> CTTTACCCTACTGGTAAATCCGCGACCTGCTC;> AAACGAGATTGAGTAAACATCGACGGATAGCTATACCGGGGGTTTCTG;> GAACCGCCCCCCCTGCCTCATTTGCCGCCAGCCGGCCAGAGGGTTACC;> GTATAAACGTACCAGGTATAGCCCGGAATAGGGTCACCAGGAATCCCCTGCGGGAT;> CTATTTCGGAACCTATGAGAAGGAGGAGGTTTGGCTGAGATTTTT;> TGATGATAAATGCCGGGAAAGGGGCTCTTCGCTATTACGCCAAGAGAA;> ATGGCTTTTAACGGGGTCAGTGCCATGACCAT;> TAAAGCCAATTCACAACCACCCTCAGAGCCGC;> CACGACGTCGTTTTAAAACGAGGCGCAGACGG;> CGGAAACATCCCGGAATTTGTGAGGGATCCCCATGCGGCGAAAGAAAC;> TGATAGACGGTTTTTCGCCCTTTGACGTTGGAGTCCACGTTCTTTAATAGTGGACTCTTGTTCCAAACTGGAACAACACTCAACCCTATCTCGGGCTATTCTTTTGATTTATAAGGGATTTTGCCGATTTCGGAACCACCATCAAACAGGATTTTCGCCTGCTGGGGCAAACCAGCGTGGACCGCTTGCTGCAACTCTCTCAGGGCCAGGCGGTGAAGGGCAATCAGCTGTTGCCCGTCTCACTGGTGAAAAGAAAAACCACCCTGGCGCCCAATACGCAAACCGCCTCTCCCCGCGCGTTGGCCGATTCATTAATGCAGCTGGCACGACAGGTTTCCCGACTGGAAAGCGGGCAGTGAGCGCAACGCAATTAATGTGAGTTAGCTCACTCATTAGGCACCCCAGGCTTTACACTTTATGCTTCCGGCTCGTATGTTGTGTGGAATTGTGAGCGGATAACAATTTCACACAGGAAACAGCTATGACCATGATTACGAATTCGAGCTCGGTACCCGGGGATCCTCAACTGTGAGGAGGCTCACGGACGCGAAGAACAGGCACGCGTGCTGGCAGAAACCCCCGGTATGACCGTGAAAACGGCCCGCCGCATTCTGGCCGCAGCACCACAGAGTGCACAGGCGCGCAGTGACACTGCGCTGGATCGTCTGATGCAGGGGGCACCGGCACCGCTGGCTGCAGGTAACCCGGCATCTGATGCCGTTAACGATTTGCTGAACACACCAGTGTAAGGGATGTTTATGACGAGCAAAGAAACCTTTACCCATTACCAGCCGCAGGGCAACAGTGACCCGGCTCATACCGCAACCGCGCCCGGCGGATTGAGTGCGAAAGCGCCTGCAATGACCCCGCTGATGCTGGACACCTCCAGCCGTAAGCTGGTTGCGTGGGATGGCACCACCGACGGTGCTGCCGTTGGCATTCTTGCGGTTGCTGCTGACCAGACCAGCACCACGCTGACGTTCTACAAGTCCGGCACGTTCCGTTATGAGGATGTGCTCTGGCCGGAGGCTGCCAGCGACGAGACGAAAAAACGGACCGCGTTTGCCGGAACGGCAATCAGCATCGTTTAACTTTACCCTTCATCACTAAAGGCCGCCTGTGCGGCTTTTTTTACGGGATTTTTTTATGTCGATGTACACAACCGCCCAACTGCTGGCGGCAAATGAGCAGAAATTTAAGTTTGATCCGCTGTTTCTGCGTCTCTTTTTCCGTGAGAGCTATCCCTTCACCACGGAGAAAGTCTATCTCTCACAAATTCCGGGACTGGTAAACATGGCGCTGTACGTTTCGCCGATTGTTTCCGGTGAGGTTATCCGTTCCCGTGGCGGCTCCACCTCTGAAAGCTTGGCACTGGCCGTCGTTTTACAACGTCGTGACTGGGAAAACCCTGGCGTTACCCAACTTAATCGCCTTGCAGCACATCCCCCTTTCGCCAGCTGGCGTAATAGCGAAGAGGCCCGCACCGATCGCCCTTCCCAACAGTTGCGCAGCCTGAATGGCGAATGGCGCTTTGCCTGGTTTCCGGCACCAGAAGCGGTGCCGGAAAGCTGGCTGGAGTGCGATCTTCCTGAGGCCGATACTGTCGTCGTCCCCTCAAACTGGCAGATGCACGGTTACGATGCGCCCATCTACACCAACGTGACCTATCCCATTACGGTCAATCCGCCGTTTGTTCCCACGGAGAATCCGACGGGTTGTTACTCGCTCACATTTAATGTTGATGAAAGCTGGCTACAGGAAGGCCAGACGCGAATTATTTTTGATGGCGTTCCTATTGGTTAAAAAATGAGCTGATTTAACAAAAATTTAATGCGAATTTTAACAAAATATTAACGTTTACAATTTAAATATTTGCTTATACAATCTTCCTGTTTTTGGGGCTTTTCTGATTATCAACCGGGGTACATATGATTGACATGCTAGTTTTACGATTACCGTTCATCGATTCTCTTGTTTGCTCCAGACTCTCAGGCAATGACCTGATAGCCTTTGTAGATCTCTCAAAAATAGCTACCCTCTCCGGCATTAATTTATCAGCTAGAACGGTTGAATATCATATTGATGGTGATTTGACTGTCTCCGGCCTTTCTCACCCTTTTGAATCTTTACCTACACATTACTCAGGCATTGCATTTAAAATATATGAGGGTTCTAAAAATTTTTATCCTTGCGTTGAAATAAAGGCTTCTCCCGCAAAAGTATTACAGGGTCATAATGTTTTTGGTACAACCGATTTAGCTTTATGCTCTGAGGCTTTATTGCTTAATTTTGCTAATTCTTTGCCTTGCCTGTATGATTTATTGGATGTTAATGCTACTACTATTAGTAGAATTGATGCCACCTTTTCAGCTCGCGCCCCAAATGAAAATATAGCTAAACAGGTTATTGACCATTTGCGAAATGTATCTAATGGTCAAACTAAATCTACTCGTTCGCAGAATTGGGAATCAACTGTTATATGGAATGAAACTTCCAGACACCGTACTTTAGTTGCATATTTAAAACATGTTGAGCTACAGCATTATATTCAGCAATTAAGCTCTAAGCCATCCGCAAAAATGACCTCTTATCAAAAGGAGCAATTAAAGGTACTCTCTAATCCTGACCTGTTGGAGTTTGCTTCCGGTCTGGTTCGCTTTGAAGCTCGAATTAAAACGCGATATTTGAAGTCTTTCGGGCTTCCTCTTAATCTTTTTGATGCAATCCGCTTTGCTTCTGACTATAATAGTCAGGGTAAAGACCTGATTTTTGATTTATGGTCATTCTCGTTTTCTGAACTGTTTAAAGCATTTGAGGGGGATTCAATGAATATTTATGACGATTCCGCAGTATTGGACGCTATCCAGTCTAAACATTTTACTATTACCCCCTCTGGCAAAACTTCTTTTGCAAAAGCCTCTCGCTATTTTGGTTTTTATCGTCGTCTGGTAAACGAGGGTTATGATAGTGTTGCTCTTACTATGCCTCGTAATTCCTTTTGGCGTTATGTATCTGCATTAGTTGAATGTGGTATTCCTAAATCTCAACTGATGAATCTTTCTACCTGTAATAATGTTGTTCCGTTAGTTCGTTTTATTAACGTAGATTTTTCTTCCCAACGTCCTGACTGGTATAATGAGCCAGTTCTTAAAATCGCATAAGGTAATTCACAATGATTAAAGTTGAAATTAAACCATCTCAAGCCCAATTTACTACTCGTTCTGGTGTTTCTCGTCAGGGCAAGCCTTATTCACTGAATGAGCAGCTTTGTTACGTTGATTTGGGTAATGAATATCCGGTTCTTGTCAAGATTACTCTTGATGAAGGTCAGCCAGCCTATGCGCCTGGTCTGTACACCGTTCATCTGTCCTCTTTCAAAGTTGGTCAGTTCGGTTCCCTTATGATTGACCGTCTGCGCCTCGTTCCGGCTAAGTAACATGGAGCAGGTCGCGGATTTCGACACAATTTATCAGGCGATGATACAAATCTCCGTTGTACTTTGTTTCGCGCTTGGTATAATCGCTGGGGGTCAAAGATGAGTGTTTTAGTGTATTCTTTTGCCTCTTTCGTTTTAGGTTGGTGCCTTCGTAGTGGCATTACGTATTTTACCCGTTTAATGGAAACTTCCTCATGAAAAAGTCTTTAGTCCTCAAAGCCTCTGTAGCCGTTGCTACCCTCGTTCCGATGCTGTCTTTCGCTGCTGAGGGTGACGATCCCGCAAAAGCGGCCTTTAACTCCCTGCAAGCCTCAGCGACCGAATATATCGGTTATGCGTGGGCGATGGTTGTTGTCATTGTCGGCGCAACTATCGGTATCAAGCTGTTTAAGAAATTCACCTCGAAAGCAAGCTGATAAACCGATACAATTAAAGGCTCCTTTTGGAGCCTTTTTTTTGGAGATTTTCAACGTGAAAAAATTATTATTCGCAATTCCTTTAGTTGTTCCTTTCTATTCTCACTCCGCTGAAACTGTTGAAAGTTGTTTAGCAAAATCCCATACAGAAAATTCATTTACTAACGTCTGGAAAGACGACAAAACTTTAGATCGTTACGCTAACTATGAGGGCTGTCTGTGGAATGCTACAGGCGTTGTAGTTTGTACTGGTGACGAAACTCAGTGTTACGGTACATGGGTTCCTATTGGGCTTGCTATCCCTGAAAATGAGGGTGGTGGCTCTGAGGGTGGCGGTTCTGAGGGTGGCGGTTCTGAGGGTGGCGGTACTAAACCTCCTGAGTACGGTGATACACCTATTCCGGGCTATACTTATATCAACCCTCTCGACGGCACTTATCCGCCTGGTACTGAGCAAAACCCCGCTAATCCTAATCCTTCTCTTGAGGAGTCTCAGCCTCTTAATACTTTCATGTTTCAGAATAATAGGTTCCGAAATAGGCAGGGGGCATTAACTGTTTATACGGGCACTGTTACTCAAGGCACTGACCCCGTTAAAACTTATTACCAGTACACTCCTGTATCATCAAAAGCCATGTATGACGCTTACTGGAACGGTAAATTCAGAGACTGCGCTTTCCATTCTGGCTTTAATGAGGATTTATTTGTTTGTGAATATCAAGGCCAATCGTCTGACCTGCCTCAACCTCCTGTCAATGCTGGCGGCGGCTCTGGTGGTGGTTCTGGTGGCGGCTCTGAGGGTGGTGGCTCTGAGGGTGGCGGTTCTGAGGGTGGCGGCTCTGAGGGAGGCGGTTCCGGTGGTGGCTCTGGTTCCGGTGATTTTGATTATGAAAAGATGGCAAACGCTAATAAGGGGGCTATGACCGAAAATGCCGATGAAAACGCGCTACAGTCTGACGCTAAAGGCAAACTTGATTCTGTCGCTACTGATTACGGTGCTGCTATCGATGGTTTCATTGGTGACGTTTCCGGCCTTGCTAATGGTAATGGTGCTACTGGTGATTTTGCTGGCTCTAATTCCCAAATGGCTCAAGTCGGTGACGGTGATAATTCACCTTTAATGAATAATTTCCGTCAATATTTACCTTCCCTCCCTCAATCGGTTGAATGTCGCCCTTTTGTCTTTGGCGCTGGTAAACCATATGAATTTTCTATTGATTGTGACAAAATAAACTTATTCCGTGGTGTCTTTGCGTTTCTTTTATATGTTGCCACCTTTATGTATGTATTTTCTACGTTTGCTAACATACTGCGTAATAAGGAGTCTTAATCATGCCAGTTCTTTTGGGTATTCCGTTATTATTGCGTTTCCTCGGTTTCCTTCTGGTAACTTTGTTCGGCTATCTGCTTACTTTTCTTAAAAAGGGCTTCGGTAAGATAGCTATTGCTATTTCATTGTTTCTTGCTCTTATTATTGGGCTTAACTCAATTCTTGTGGGTTATCTCTCTGATATTAGCGCTCAATTACCCTCTGACTTTGTTCAGGGTGTTCAGTTAATTCTCCCGTCTAATGCGCTTCCCTGTTTTTATGTTATTCTCTCTGTAAAGGCTGCTATTTTCATTTTTGACGTTAAACAAAAAATCGTTTCTTATTTGGATTGGGATAAATAATATGGCTGTTTATTTTGTAACTGGCAAATTAGGCTCTGGAAAGACGCTCGTTAGCGTTGGTAAGATTCAGGATAAAATTGTAGCTGGGTGCAAAATAGCAACTAATCTTGATTTAAGGCTTCAAAACCTCCCGCAAGTCGGGAGGTTCGCTAAAACGCCTCGCGTTCTTAGAATACCGGATAAGCCTTCTATATCTGATTTGCTTGCTATTGGGCGCGGTAATGATTCCTACGATGAAAATAAAAACGGCTTGCTTGTTCTCGATGAGTGCGGTACTTGGTTTAATACCCGTTCTTGGAATGATAAGGAAAGACAGCCGATTATTGATTGGTTTCTACATGCTCGTAAATTAGGATGGGATATTATTTTTCTTGTTCAGGACTTATCTATTGTTGATAAACAGGCGCGTTCTGCATTAGCTGAACATGTTGTTTATTGTCGTCGTCTGGACAGAATTACTTTACCTTTTGTCGGTACTTTATATTCTCTTATTACTGGCTCGAAAATGCCTCTGCCTAAATTACATGTTGGCGTTGTTAAATATGGCGATTCTCAATTAAGCCCTACTGTTGAGCGTTGGCTTTATACTGGTAAGAATTTGTATAACGCATATGATACTAAACAGGCTTTTTCTAGTAATTATGATTCCGGTGTTTATTCTTATTTAACGCCTTATTTATCACACGGTCGGTATTTCAAACCATTAAATTTAGGTCAGAAGATGAAATTAACTAAAATATATTTGAAAAAGTTTTCTCGCGTTCTTTGTCTTGCGATTGGATTTGCATCAGCATTTACATATAGTTATATAACCCAACCTAAGCCGGAGGTTAAAAAGGTAGTCTCTCAGACCTATGATTTTGATAAATTCACTATTGACTCTTCTCAGCGTCTTAATCTAAGCTATCGCTATGTTTTCAAGGATTCTAAGGGAAAATTAATTAATAGCGACGATTTACAGAAGCAAGGTTATTCACTCACATATATTGATTTATGTACTGTTTCCATTAAAAAAGGTAATTCAAATGAAATTGTTAAATGTAATTAATTTTGTTTTCTTGATGTTTGTTTCATCATCTTCTTTTGCTCAGGTAATTGAAATGAATAATTCGCCTCTGCGCGATTTTGTAACTTGGTATTCAAAGCAATCAGGCGAATCCGTTATTGTTTCTCCCGATGTAAAAGGTACTGTTACTGTATATTCATCTGACGTTAAACCTGAAAATCTACGCAATTTCTTTATTTCTGTTTTACGTGCAAATAATTTTGATATGGTAGGTTCTAACCCTTCCATTATTCAGAAGTATAATCCAAACAATCAGGATTATATTGATGAATTGCCATCATCTGATAATCAGGAATATGATGATAATTCCGCTCCTTCTGGTGGTTTCTTTGTTCCGCAAAATGATAATGTTACTCAAACTTTTAAAATTAATAACGTTCGGGCAAAGGATTTAATACGAGTTGTCGAATTGTTTGTAAAGTCTAATACTTCTAAATCCTCAAATGTATTATCTATTGACGGCTCTAATCTATTAGTTGTTAGTGCTCCTAAAGATATTTTAGATAACCTTCCTCAATTCCTTTCAACTGTTGATTTGCCAACTGACCAGATATTGATTGAGGGTTTGATATTTGAGGTTCAGCAAGGTGATGCTTTAGATTTTTCATTTGCTGCTGGCTCTCAGCGTGGCACTGTTGCAGGCGGTGTTAATACTGACCGCCTCACCTCTGTTTTATCTTCTGCTGGTGGTTCGTTCGGTATTTTTAATGGCGATGTTTTAGGGCTATCAGTTCGCGCATTAAAGACTAATAGCCATTCAAAAATATTGTCTGTGCCACGTATTCTTACGCTTTCAGGTCAGAAGGGTTCTATCTCTGTTGGCCAGAATGTCCCTTTTATTACTGGTCGTGTGACTGGTGAATCTGCCAATGTAAATAATCCATTTCAGACGATTGAGCGTCAAAATGTAGGTATTTCCATGAGCGTTTTTCCTGTTGCAATGGCTGGCGGTAATATTGTTCTGGATATTACCAGCAAGGCCGATAGTTTGAGTTCTTCTACTCAGGCAAGTGATGTTATTACTAATCAAAGAAGTATTGCTACAACGGTTAATTTGCGTGATGGACAGACTCTTTTACTCGGTGGCCTCACTGATTATAAAAACACTTCTCAGGATTCTGGCGTACCGTTCCTGTCTAAAATCCCTTTAATCGGCCTCCTGTTTAGCTCCCGCTCTGATTCTAACGAGGAAAGCACGTTATACGTGCTCGTCAAAGCAACCATAGTACGCGCCCTGTAGCGGCGCATTAAGCGCGGCGGGTGTGGTGGTTACGCGCAGCGTGACCGCTACACTTGCCAGCGCCCTAGCGCCCGCTCCTTTCGCTTTCTTCCCTTCCTTTCTCGCCACGTTCGCCGGCTTTCCCCGTCAAGCTCTAAATCGGGGGCTCCCTTTAGGGTTCCGATTTAGTGCTTTACGGCACCTCGACCCCAAAAAACTTGATTTGGGTGATGGTTCACGTAGTGGGCCATCGCCC;> TTCGCCATTCAGGCTGCCAGCTTTTTTTT;> TCGATGAACGGTAATCAAGCGCCAGGCGATCGCAGTTTGATTCTAGCT;> TTTTTGGAGCAAACTACAAAGCATTGCCTGCTATTTTAAAAGGGTGAGAAAGG;> TTTTCCGGCACCTCGGCCTCAGGAATTTTTTTTTTGATCGCACTCCAGGGTCAGGATTTT;> ACCAGGCAGGATAGGTGCATCTGCTCCTGTAGTTTTAAATGCAATGCC;> ATCAGCTCGTAAAACTTCAGAAAAGTGCGGGCGATGTGCTGCAAGGCG;> TTTTCCGTGGGATTAAATGTGAGCGTTTTTTTTTTAGTAACAACCCGTTTTTGATATTTT;> ACCAATAGGAACGCCATTTTGTTATTTTTTTTTTAAATTCGC;> TTTTCAACTAAAATATAATGCTGTATTTTTTTTTTGCTCAACATGTTTAGAGCTTATTTT;> TCTGGAAGTTTCATTCATAGTAGTGCAAAGAA;> AGCATTAACATCCAATATTTGGGGTTTTTTTTCGCGAGCT;> TAGTTTGATTAGCAAAAATCGGTTGTACCAAACTACAGAGTAAAATGT;> CCATTAGAGCAAGGATAAAAATTTGGTAATAG;> TCAATAACATATTTTCAATACTTTTCCACAGAGAAAGACAGCATCGGA;> CATCAACAACAAACGGCGGATTGACCGTAATGCATATAAC;> CCAGCTTTAGTAGATTAGTTGATTCCCAATTCTAAATATGTTTTT;> TCAAAAATGCAAATGGGAAAAGGTGGCATCAATTCTACTAATTTTTTA;> AAGCAAATCGTTAATAAAAGATTCTGCGGGAGCCAATACTGCGGAATC;> GGGGACGAGTAACCGTCACGTTGGTGTAGATGCGGATTCTTTTTT;> CCACCACCGCAGGTCAGACGATTGTTTGCTCAAGTTAATGCTCAAATG;> CACCAGAAAACCTCACAGCGCAGTCGCAGAAACAGCGGAT;> TTTTTGCCACCCTAACCGCCTCCCTCTTTTTTAGAGCCGCCACCCCCAGAGCCTTTTT;> TTTTTTAGAGAGAACCAGACCGGAATTTTTTTTTTGCAAACTCCAACAGAACGAGTTTTT;> TACCTTTAGGGTAACGCGCAACTGTTGGGAAG;> GATAAATTCAGGAGTGTGTAAAACACGGTGTACAGACCAGATCTTGAC;> AGAGGGTAGTACCCCGGATTGTATATTAAATTTTTGTTAA;> AGGTTGAGAGAGCCGCCGCCAGCATGAGAGATCTTTCAGACGTCATAC;> CACCATCAAAATATCGTGACTATTATTATACCAAGCGCGA;> CCGGAGACAACAGGAAGTTGATAAAGCATGTCAATCATATGAGAGTCTTTTTT;> CGGATAAGTGCCGTCGTTGACAGGCCAGTAAGGGTGGAGC;> TTAGGATTAGCGGGGTGCCTTGATGAATGGAA;> TTTTTCTCCTCAATATTCTGAAACATTTTTTTGAAAGTATTAAGATTGCCATCTTTTT;> TTTTAGAGGTCACGGATTGCATCAATTTTTTTTTTAAAGATTAAGAGGACGGAACATTTT;> TTTTTGCGATTGCTCCGGCGCATCCGACAGTAGCTTCTGGTGCCGGAA;> ATTTCAACTACATTTCAATTCGCGTCTGGCCTGCCCCAAAAGTCAAAT;> AAGCCTTTGACCCTGTAAATCATACAGGCAAG;> TACAAACTATAGTTAGCGTAACGATTGAAAATGCCGCTTTATGACAAC;> TTTTTATAGGAACGCCACCACCCTCATTTTTTTTTTCAGGGATAGGGCATTTTTTTTT;> TTTTATTGCTGAAAAATAGCGAGAGTTTTTTTTTTGCTTTTGCAAAAGGACGACGATTTT;> TTTTCTAAAGGAACAGTTTCAGCGGTTTTTTAGTGAGAATAGAACCTTTAGCTTTTT;> TTTTAGCCTTTATAACCGATATATTTTTTTTTTTTCGGTCGCTGAGGCGTCTGGTCTTTT;> AGCTTGCTTTCGAGGTCGCCGACATGGGATTTTGCCGGACAGAGCACA;> CCCACGCAATTGTATCAAAAGGCTCCAAAAGGTTTTT;> GATAGTTGGAATTTCTTAATAATTTTTTCACGTCTAAAGT;> TGCTAAACAACTTTCAATTGCGAATAAACAGCAGGAACAATTTT;> GCTTTGAGTAAACGGGTAAAATACCGCCAAAACATTCAAC;> TCAGCAGCCAGCCCTCACAACGCCTGTAGCATAGAGGGTT;> TTTCTGTAACCCTCAGGTTAAACGATGCTGATCAGATGCCTTGCCCTGTTACCAGA;> AAATGAATTTTGTCGTCGTAACACTGAGTTTCTGTATCAC;> CCAGAGGGTTAGAACCTAAAGCTAATTAAGCAATAAAGCCGTACGGTG;> AACCGCCACCCTCAGACCATGTACCTTTCCAGCAAGCCCATTTTT;> TTTATTACGCATCAAAAATGAAAATTTTTTTTTTTAGCAGCCTTTACTCTTTCCTTTTTT;> TTTTGGGTGCCTCCATCACCCAAATTTTTTTTTTTCAAGTTTTTTGGGCAAACTATTTTT;> CACATTAATTGCGTTGAAACAGGGTAAGAAACACCAAGTA;> CGCTCACTGCAAACGTAGGGAGGGAAGGTAAA;> GTCGTGCCGAACAAAGCGGCTGGTAATGGGTA;> TTTTACCCAAAACTGAACACCCTGATTTTTTTTTTACAAAGTCAGAGGAATAAGAGTTTT;> TTTTTCGGCCAACGTTCCAGTACTCCAACAATCGTCTGAAATGGAAAACATCG;> AAGTAAGCCAAAAGAATTGCAGCATAACCTCCGGCTTAGGCAAATCCA;> TTTAAGAAAGGAAACCGAGGAAACGCCCGCTT;> AAGCCCTTTCGATAGCAGCACCGTGTAGCGCGCCACGCAATTGATACC;> ATCGGCGAAACGTACACAGAGCCAACAAATAATCAGAACCTTTTT;> ACAGATGAGACGGCCAGTGCCAAGCAGCTGGC;> TGGTGAAGCCAACTTTTTCTTCGCGTCCGTGACACACAACTTTTT;> TTTTTACCACCGGTAGAAAATTCATATTTTTTTGGTTTACCAGCGATTTTGTCTTTT;> TTTTTAGTAAATTAAGGCTTGCCCTGTTTTTTTTTTACGAGAAACACCAACCTTCAT;> CGAACTGATCATCGCCGTCACTGCGCGCCTGTAAAGCCTGTTTTT;> ATCAAAATATTAGCGTAGTACCGCCACCCTCACGTACTCA;> TTTTTTTTTCATATATTGACGGAAATTTTTTTTATTCATTAAAGGGACTCCTTTTTT;> TTTTTACATTATTAAAATCTACGTTATTTTTTTTTTATAAAACGAACTAAATTTCAA;> GATTTGTACCTAAAACCACTGGTGTGTTCAGCTAATGAATTTTTT;> CGCACAGGCGGCCTTTAGTGATGAAATTTCTG;> TCTTTGACGTTTCCATGACTAAAGACTTTTTCTCAGAGCAGATGGCTTTGCGAACG;> TACACTAAAACACTCAGAATACCAGGAATTAC;> GAAAGAGGACTACGAAACGAGGGTAGCAACGGAACATTAT;> GCGGTCCGATAAAAAAGGTGCCCCCTGCATCAGACGATCCATCCCTTA;> TTTTTCGGTCATAAAAATCACCAGTATTTTTTGCACCATTACCATAACGGAATTTTTT;> TTTTTTAAAAACCAACACTATCATAATTTTTTTTTTCCCTCGTTTACCAATCAGTTG;> GTAATGCCCAAAAGAATTAGACTGAATCAGGTTGAGTAATGTGTAGGT;> GGCACCAATTTTTTCGAAGGTTTCTTTGCTCGTCATAAACATACATAA;> TCTCGTCGCTGGCAGCCGTCACCCAGTTAAAGCTCCAAAAGGTTTATC;> CTCCGGCCTTGTAGAAGGTCACTGGCATCAGCTTCACCAGTGAGACGG;> TTTTTGTCAGACTAATCAGTAGCGACTTTTTTAGAATCAAGTTTGGAAATAGCTTTTT;> TTTTAGCAGCAACTTTCGCACTCAATTTTTTTTTTTCCGCCGGGCGCGTTTGCGTATTTT;> GGCAGCACCGTCGGTGGGTGTCCATGAAACCA;> GGGGTCATTGCAGGCGCCGCAAGATGGTGCTGTTGCAGGG;> GTTGCGGTATGAGCCGCGTCAGCGATGCCAACAACCATCG;> GAGGCATAGTAAGAGCATGAGGAAAAAGATTCAAGTTTTGAAGCAAAG;> GTCACCAAAGCCATTTTCCAGTCGGGAAACCTCCGTCTATTAGCCCGA;> TAGCAAGGCCGGAAACTCCTCATAAGGGTAAA;> TAATGCAGTAAGAACTAACAAAGTACAACGGAAAATCAAAGATAGCGT;> AAATCGTTGCGGTGCCATCCCGTAAAAAAAGCCTTTAAACTATTCATT;> AACGGCATTGCCGTTCCGGCAAACGTCATAAAAGTTCAGAGATATAAG;> GGGAATTAGAGCCAGCGCCCCCTTTTTTCATCACGTTAGT;> TGGGAAGAACAGGTAGGATGGTTTAAGCCCGAAAGACTTCATATGATACTCATATA;> GGCTCATTTTACCTTATGCGATTTTTACCCAATCAATCAT;> CCGACTTGACCGATTGAGAAAATACATACATA;> ATTGTGAAATACCAGTCAGGACGTAGATTTAG;> GCACTCTGTCACGGTCCTCACGGATTTCTCCGCGCCACGGGAACGGAT;> CAGTGAATGGGCTTGAGCTGGCTGCCAGGGTTTTCCCAGTATTAAGTTTTCAACCG;> AACAAAGCTGCTCATTCTTTAATCCATGTTACCCCCAGCGATAGTCAG;> ATCAACGTAAGAACCGGATATTCACGTGCCTGGAAAGAGGAAGGGAAC;> CCAGCACGAGCGCAGTTGATAAATTGTGTCGAATAAGTTT;> GGCCGTTTTGGTGCTGAGTTGGGCGGTTGTGTCAGTGCCCTTACCGTT;> GACATTCAGGGTACCGTCCTGTGTGAAATTGTGGAAGGGATCGGAACC;> CCAAAGACAAAAGGGCCAAACTTATTTACCAG;> CAAGAGTAGCGCATAGTTAGCCGGTTCGAGCTTCAAAGCG;> GCCTCCTCACAGTTGAAGATAGACAAAAGAGACTCTGAAT;> AGCTCGAATTCGTAATGCGCCATGCACCGGAAATCCTCAT;> TTTACAATCAATAATTTGCCAGTTTTTTTTTTTTACAAAATAAACAGGCGTCTTTTTTTT;> TTTTTATACGAGCATTTAGAGAAAGCCGGCCGCGCTTAATGCGCC;> GCAAAGACAATCCAAAAGAAAGCGAGCGGTCACGCTGCGC;> GTATGTTAATGATTAATGAATTATCACCGTCA;> TTTTTCCAGAGCCATCCTGAATCTTATTTTTTTTTTCCAACGCTAACGAGCGCCCAA;> TTTTTGTAAAAGATGAGAAGTGTTTTTTTTTTTTTTTATAATCAGTGAGTTTCCTCG;> GTAATAACATCACTTGAAGAACGCAGGTTTTG;> CCTGAGTACACACCCGCGAACGTGGCGAGAAATATCCGCTAACATATA;> CCGTTTTTCCGCACTCGAAAAATAAATAAACAACATGTTCTAATTGAG;> ATTTTCATAAATCAGATATTTTGCACCCAGCTACAATTTTGGGCGCTG;> CGTAGGAAGCAAGTGTAAAGGAGCGGGCGCTACATGGTCAATAAGTTT;> TCATTACCCCATATTATTTATCCCACCACGGATAGCTGTT;> ATCGAGAAATCCAGAATGGCCCACTACGTGAAAATGAGTGTAAAGTGT;> TTTTTTATCATTCTGTAGAAACCAATTTTTTTTTTTCAATAATCGGCTGAAGTAATT;> TCTTACCGTGATTGCCCCAGCTTACGGCTGGAGTGCCATCACGGAACG;> TTTTAATAGCTAGCCCAATAATAAGTTTTTTTTTTAGCAAGAAACAATAATACCGATTTT;> TTTTTTTGGGCGCTTGCCCCAGCAGGCGAATCAAAAT;> GGTTTAACTGTTTGGATTATATTTTTTTTTTCTTCTGAATAATGTCAATATATTTTT;> AGCGGTCCACGCTGGTCAGGGTGGAGAGGCGG;> TGAGAGAGGATAACCCTAAGAATAAACACCGGAACTTTTT;> TGCACGTATAATACATTTGAGGATTAGAGCCG;> AAATCGGCAAAGAAACCACCAGAAATAGCGATGTGAATTTTAGAATCCTTTTT;> AAAATCCCTTATAAATAGATAGCCTTTTTCTT;> TTACAAACTTGAGGAAGGTTATTTTTTTTTTTCTAAAATATCTTCAACAGTTTTTTT;> ATTAGACTAGAACCTACCATATCAATTGCGTA;> ATCAGAGAAAGCGCATACGCTCATGGAAATACAATCGCCA;> TAGACGGGAGAATTAAGAACTGGCGCAATAAT;> TAAAAGGGTAGGAGCACTAACAACTAATAGATTTAGAAGTTTAAATCCTGATTATC;> ATTCACCAGTCACACGAGATAGAACACCGCCTTGAAAAATCTGAGCAA;> CTACATTTTTACTAGAGATAGGGTTGAGTGTTGCGCGGGGAGCTGCAT;> TTTTTAATATAAATTAGGCAGAGGCATTTTTTTTTTTTTTCGAGCCAGTAATTCTTA;> TTTTGAAAGGAAAATCAATATCTGGTTTTTTTTTTTCAGTTGGCAAATCAAATATCTTTT;> TTTGCCCGAGTATTAACCCTTCTGATATTTTTCTAAAGCATCACCTTG;> AACGTTATATTGGCAGTCAATAGACTATTAAAGAACGTGGTTGGAACAAAAGTTTG;> AGTAACATCCAGCAGAAGATAAAACGAACTGATTTTT;> TATCATTTTGACGCTCGTCAAAGGGCGAAAAA;> AAAAGCCTGTTTAGTAAAGCCAACTATTTAAC;> TTTTTCCGTGTGACTTCTGACCTAAATTTTTTTTTTTTTAATGGTTTGATATGTAAA;> TTTTATCCTGATAAATTAATTACATTTTTTTTTTTTTAACAATTTCATAAACATCATTTT;> GTAACAGTACCTTTTATGCTTTGACAGTACATCTGTAAATGAATGGCT;> GAAACAATAAATCCTGAAACAGAAATAAAGAAAAATTATTCATATTCC;> CATAGGTCAGTCAATAAGCTTAGATTAAGACGACGAACCA;> TCGCGCAGGTCAGATGAATATACAGATTTTCA;> ATCGCAAGACAAAGAACTGAGAAGTGAGAGACTGCGGAAC;> TGCTGATGTTGGGTTAGCGTTAAAACAAGAATTGAGTTAA;> CCTTTTTTAGATGATGGCAATTCAGAAGGGTT;> AATGGAAAATACCAAGTCAATTACCGTCGCTATTAATTAA;> CAAATATATTTTAGTTCCAGTATATCATATGCCAGGAAAA;> AATTTCATTAAATAAGTATAACTACTTCACCGCCTGGCCCGCAACAGC;> GCTCAACAGTAGGGCTCGCGAGAAAATCATAATACCTTTT;> GCGTAAGATTATTTACTAATTTTAAGAGTCCATTTGATGGTGGTTCCG;> CCATTAAAAATACCGAAGCTAATGCTGGTAATGAAGAACT;> AACGCCAACTGTCCAGCATTGCAAGGTATTAAGATTTTTTGTTTAACG;> CATGTAATGTACCGACGTTATACAGTAATTGAGCGCTAAT;> CTGAACCTACATTCTGGCCAACAGACCAGTAAAACTCGTA;> TTTTTTAGCCCTAATACGTGGCACAGACAACCTGAAA;> TTTTTAAACCCTCGAGAGCCAGCAGCAAAGCAACAGT;> ATTAGTCTTTAATGCGCAGAGGTGATATGTGAGGAGCGGA;> AAGAAGATGATGAAACTTGAATTAGCCACGCTAATTCGAC;> TTTTTTTGAAAACGTGAATAACCTTGCTTAAATCAATAGGCGGTC;> TTTTTAGAAAACAAGGCGAATTATTCATTTTACAAAA;> TTTTCCCTAACGGATTCGCCTGATCATCGGGAATTATCAT;> GTCGAGGTGCCGTAAAAAGGTGGCAGCTAACTTGCAGCCA;> GCACTAAACAGGGCGACAATATTACCGCCAGC;> CTAAAGGGAGCCCCCGCGGAAGCACACAATTC;> TATGGTTGCTTTGACGAGAGCGGGGACAGGAA;> TTTTTCGGCCTTGCAGAACGCCAACAATAGATAAGTCGGTATTCT;> ACGACGACATATCCCATCCTAATTTAGCAAGC;> TACGAGCACAAGAACGAAAAGGTAAGAGAGAATAACATAA;> CGGTACGCCAGAATCCGTCTGTCCTAACGTGCGCCACCGATTTTT;> TTAGAATCAGCACGTAATCACGCAAATTAACCGTTGTAGCGGATTTTA;> AGCTAAACAGGAGGCCCCTCCCGAGCTACAGGTTTGATTA;> CTTGCGGGGAGGCGTTTTAGCGAAGATTAAAGAATACTTCGCGCGTAC;> AAGCCTTAAATCAAGAGTAACCACCAAGCAAG;> TTAGTTGCTATAGAAGGCTTATCCCTGAACAA

Here, we addressed the problem of accurate structural validation with cryo-EM-based methodologies for determining the structures of up to megadalton-scale DNA objects in solution, together with molecular-dynamics-based methods for building pseudoatomic models in a semiautomated fashion. The library of objects includes four brick-like multilayer DNA origami objects with increasing internal floppiness, a barrel-like 126-helix bundle, two variants of a multidomain object called Twisttower, a design variant v2 of a previously reported object called the Pointer, a small 16-helix bundle, four variants of a hinged-beam-like object, two variants of a dumbbell-like object, and five variants of a six-helix tube featuring asymmetric markers at either end as reporters for twist and one ten-helix tube. We constructed pseudoatomic models for six different objects. The fitting was validated using Fourier shell correlation against the cryo-EM half-maps and the models show good cross-correlation with the cryo-EM maps.

The object termed Twisttower is a complex of four cuboid-like domains fused together. The cuboids feature 2 × 2, 4 × 4, 6 × 6, and 8 × 8 helices, respectively, in a quadratic cross-sectional arrangement. In the cryo-EM map that we determined, each cuboid domain exhibited an independent right-handed twist deformation around the helical axis of the domain. Such twist deformations are expected to arise a priori for square-lattice designs with default eight-base-pair crossover spacing because the design specifics create right-handed internal torques. The global twist observed in each Twisttower domain decreased with the increasing cross-sectional area (left). Exemplarily, we found that the Twisttower samples an ensemble of conformations in which the different domains move relative to each other by bending and twist deformations at the domain interfaces. In particular, the 2 × 2 and the 4 × 4 domains show relative displacements with up to 12-nm (extreme to the extreme) amplitude (Fig. 3a and Supplementary Movie M1). A Frankenstein map of the Twisttower (bottom), which is generated by merging the maps from the different focused refinements, allows appreciating that now virtually all parts of the Twisttower are resolved with high detail.>MPSKKNGRSGPQPHKRWVFTLNNPSEDERKKIRDLPISLFDYFIVGEEGNEEGRTPHLQGFANFVKKQTFNKVKWYLGARCHIEKAKGTDQQNKEYCSKEGNLLIECGAPRSQGQRSDLSTAYSDYQQSDPVGMVLLNCCPSCRSSLSEDYF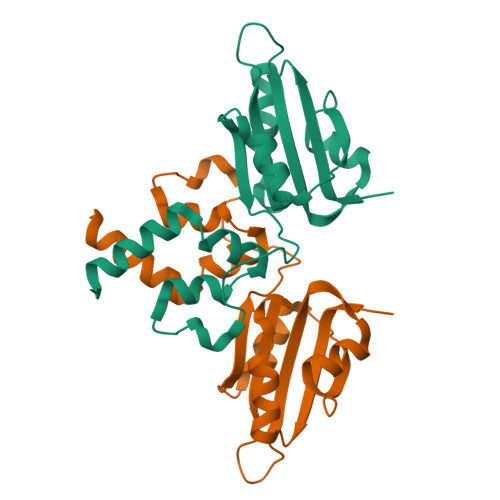LGILEECYRTIHGGRGPVRHPFPPMPLEHHHHHH[2x]>[2x]MHHHHHHSSGRENLYFQGASTSAVMSCTLGKATCLGMDKICSPLADNDVTQRKTQIICTIGPSCNNVESLIGLI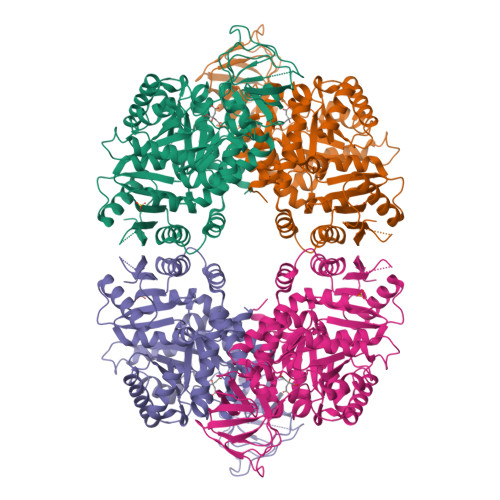DKGMSVARLNFSHGDHESHFKTLQNIREAAKARPHSTVGIMLDTKGPEIRTGMLEGGKPIELKAGQTLKITTDYSMLGNSECISCSYSLLPKSVQIGSTVLIADGSLSTQVLEIGDDFIVCKVLNSVTIGERKNMNLPGCKVHLPIIGDKDRHDIVDFALKYNLDFIALSFVQNGADVQLCRQIISENTQYSNGIPSSIKIISKIENLEGVINFDSICSESDGIMVARGDLGMEIPPEKIFVAQKCMISKCNVAGKPVVTATQMLESMIKSNRPTRAEMTDVANAVLDGSDCVMLSGETANGAFPFDAVNVMSRVCAQAETCIDYPVLYHAIHSSVPKPVAVPEAIACSAVESAHDVNAKLIITITETGNTARLISKYRPSQTIIACTAKPEVARGLKIARGVKTYVLNSIHHSEVVISNALALAKEESLIESGDFAIAVHGVKESCPGSCNLMKIVRCP> XPPPV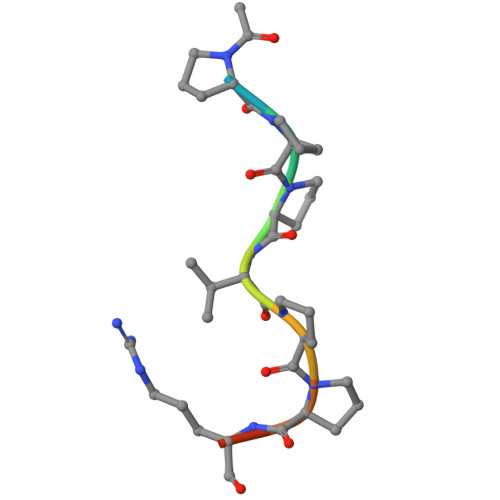PPRRR> MAETRDQVKKLQLMLRQANDQLEKTMKDKQELEDFIKQSSEDSSHQISALVLRAQASEILLEELQ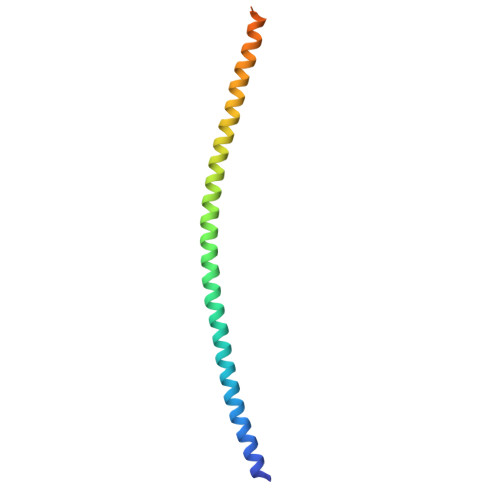QGLSQAKRDVQEQMAVLMQSREQVSEELVRLQKDNDSLQGKHSLHVS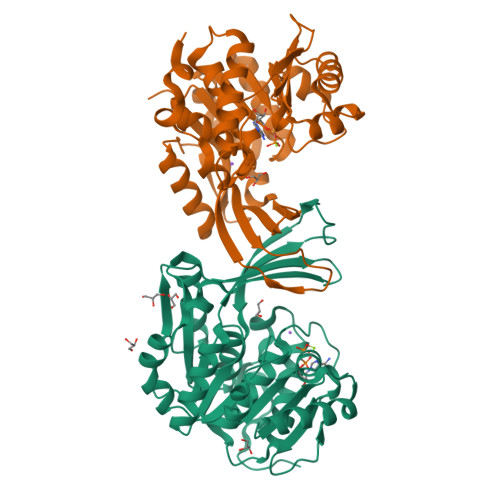>EVAAVVVVGSCMTDLVSLTSRLPKTGETIHGHKFFIGFGGKGANQCVQAARLGAMTSMVCKVGKDSFGNDYIENLKQNDISTEFTYQTKDAATGTASIIVNNEGQNIIVIVAGANLLLNTEDLRAAANVISRAKVMVCQLEITPATSLEALTMARRSGVKTLFNPAPAIADLDPQFYTLSDVFCCNESEAEILTGLTVGSAADAGEAALVLLKRGCQVVIITLGAEGCVVLSQTEPEPKHIPTEKVKAVDTTGAGDSFVGALAFYLAYYPNLSLEDMLNRSNFIAAVSVQAAGTQSSYPYKKDLPLTLFLEHHHHHH[2x]> IL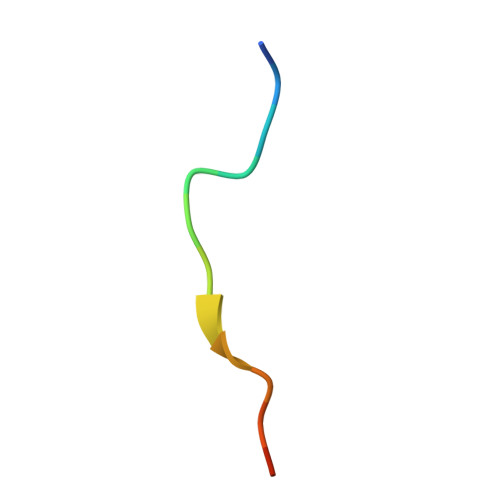AWGRGGTRSNTR>MKHHHHHHQGKITLYEDRGFQGRHYECSSDHPNLQPYLSRCNSASVDSGCWMLYEQPNYSGLQYFLRRGDYADHQQWMGLSDSVRSCRLIPHSGSHRIRLYEREDYRGQMI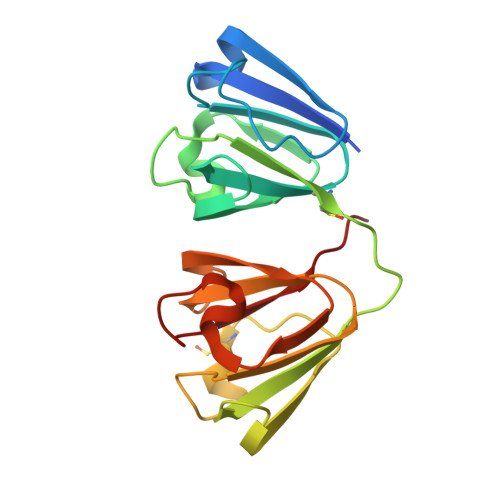EFTEDCSCLQDRFRFNEIHSLNVLEGSWVLYELSNYRGRQYLLMPGDYRRYQDWGATNARVGSLRRVIDFS[2x]> TGQKLDDVDPLVATNFGKIRGIKKELNNEILGPVIQFLGVPYAAPPTGERRFQPPEPPSPWSDIRNATQFAPVCPQNIIDGRLPEVMLPVWFTNNLDVVSSYVQDQSEDCLYLNIYVPTEDDIRDSGGPKPVMVYIHGGSYMEGTGNLYDGSVLASYGNVIVITVNYRLGVLGFLSTGDQAAKGNYGLLDLIQALRWTSENIGFFGGDPLRITVFGSGAGGSCVNLLTLSHYSEGLFQRAIAQSGTALSSWAV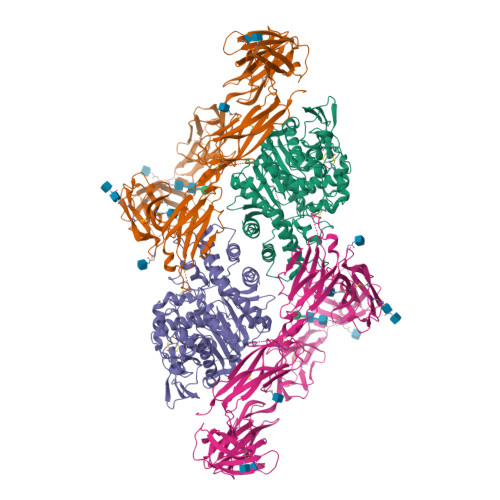SFQPAKYARMLATKVGCNVSDTVELVECLQKKPYKELVDQDIQPARYHIAFGPVIDGDVIPDDPQILMEQGEFLNYDIMLGVNQGEGLKFVENIVDSDDGISASDFDFAVSNFVDNLYGYPEGKDVLRETIKFMYTDWADRHNPETRRKTLLALFTDHQWVAPAVATADLHSNFGSPTYFYAFYHHCQTDQVPAWADAAHGDEVPYVLGIPMIGPTELFPCNFSKNDVMLSAVVMTYWTNFAKTGDPNQPVPQDTKFIHTKPNRFEEVAWTRYSQKDQLYLHIGLKPRVKEHYRANKVNLWLELVPHLHNLNDRTKHHHHHH;> QGVYAPAQAQIIHAGQACVVKEDNISERVYTIREGDTLVLQCLVTGHPRPQVRWTKTAGSASDKFQETSVLNETLRIEKIQRLQGGRYYCKAENGVGVPAIKSIRVDVQYLDEPVLTVHQTISDVRGSFYQEKTVFLRCTVNSNPPARFIWKRGAETLSHSQDNGVDIYEPLYTQGETKVLKLKNLRPQDYASYTCQVSVRNVCSIPDKSITFQLTNTTAPPALKLSVNETLVVNPGDNVTMQCSLTGGDPQPEVLWSHSPGPLPPNSLVQGGNLTIWRIRVEDSGYYNCTAINNVGNPAKKTVNLLVRSMKNATFQITPDVIKESETIQLGQDLKLSCHVDAVPQEKVVYSWYKNGKPARFSDRLLITRNDPELPPVTCSLEIIDLRFSDYGTYLCVATFQGAPIPDLSVEVNISSETVPPTISVPKGQSTITVREGSRAELQCEVRGKPKPPIIWSRVDKETPMPSGTMTVETYDGKLRLESVSRDMSGTYKCQTARYNGFNIRPREALVQLNVQFPPVVEPAFQDVRQGMGRSVTLRCTMLKGSPMKVATSVWRFNGTLLAQPPAEQQDYSELKVDSVSRETSGSYECSISNDVGVSACLFQVSAKAYSPEFYYDTPNPTLSQKQSKNYSYILQWTQKEPDAVDPILKYRLEVRQLAQRNTIQTFIPVQKMEKGLLLEHILPNLKVPQSYEVRLTPITSFGAGDMAARIIRYMEPINYPSPTDNTCRFEDEKICGFVQDKMDNFDWTRQNALTQNPKRTVNTGPPTDISGTPEGYYMFIEASRPRVTGDKARLISPLYNITAKYYCVSFYYHMYGKHIGSLNLLVRVRNKRAIDTQVWSLSGNRGNMWQQAHVPINPPGPFQIIFEGVRGTSYEGDIAIDDVTLKKGDCPRKPIGPNKGTKHHHHHH> NSHQK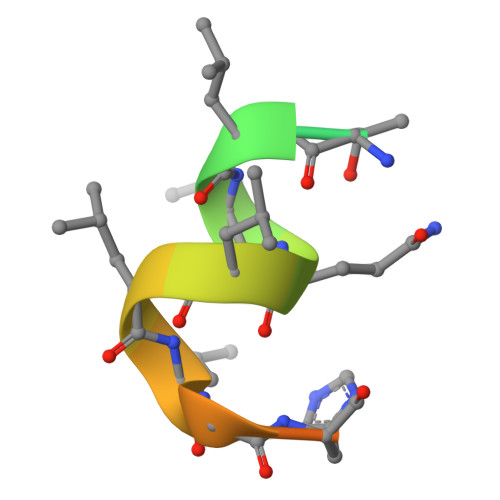VTLLQLLLGHKNEEN>MHHHHHHSSGMSDKIIHLTDDSFDTDVLKADGAILVDFWAEWCGPCKMIAPILDEIADEYQGKLTVAKLNIDQNPGTAPKYGIRGIPTLLLFKNGEVAATKVGALSKGQLKEFLDANLAGTENLYFQSMKKKVWREEKERLLKMTLEERRKEYLRDYIPLNSILSWKEEMKGKGQNDEENTQETSQVKKSLTEKVSLYRGDITLLEVDAIVNAANASLLGGGGVDGCIHRAAGPCLLAECRNLNGCDTGHAKITCGYDLPAKYVIHTVGPIARGHINGSHKEDLANCYKSSLKLVKENNIRSVAFPCISTGIYGFPNEPAAVIALNTIKEWLAKNHH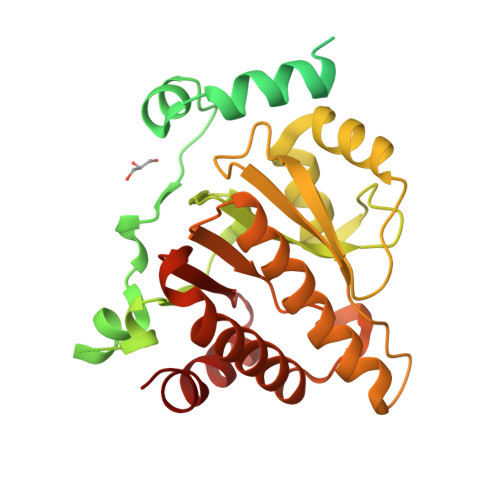EVDRIIFCVFLEVDFKIYKKKMNEFFSVD[8x]>MALSQATDPFRAAVEFTLMPMLITNPHLPDNPIVFANPAFLKLTGYEADEVMGRNSRFLQGHGTDPAHVRAIKSAIAAEKPIDIDIINYKKSGEAFWNRLHISPVHNANGRLQHFVSSQLDVTLELSRLVELEKERKTLSIEHHHHHH[4x]

LOV-HK is a blue light photoreceptor from Brucella abortus, a pathogenic α-2-proteobacterium that can be transmitted from cattle to humans causing brucellosis. B. abortus LOV-HK comprises an N-terminal blue light-sensing LOV domain, a central PAS (Per-Arnt-Sim) domain of unknown function and a C-terminal HK domain. The LOV and PAS domains are connected through a long linker helix denoted the Jα helix, while the HK domain belongs to the HWE family. Upon blue light illumination, B. abortus LOV-HK photobleaches as a result of the adduct formation between its flavin mononucleotide (FMN) chromophore and an adjacent conserved cysteine residue as in other LOV proteins.

The blue light sensing LOV domain is flanked by α helices at both its N and C termini, denoted the Nα and Jα helices, respectively. We crystallized and obtained the structure of a “blind” construct consisting of the Nα helix, half of the Jα helix, and the LOV core (LOVN13J21 C69S). The structure reveals a parallel dimer, in which the Nα helices intertwine and interact with the β sheet of the core. Such dimeric association is similar to those observed in other LOV and PAS domains, but it contrasts with the isolated core of the LOV domain, which forms an antiparallel and unstable dimer. The Nα helix plays a central role in the dimer formation, interacting with the hydrophobic β-sheet. In contrast, the addition of the Nα helix (LOVN13J21 construct) strongly promotes the dimer formation. In addition, the presence of the Nα helix dramatically increases the lifetime of the light state in LOVN13J21, with no detectable decay for at least 30 h after light excitation, while the light states of both LOVJ5 and LOVJ20 slowly decay in hours. Taken together, these results demonstrate that the Nα helix plays an essential role in forming a parallel dimer.In the bloodstream an unusually tight interaction between the bacteria and the brain microvasculature endothelial cells is established, leading to cortical plaque formation that results in opening of the blood brain barrier and bacterial invasion of the brain. This interaction is mediated by Type IV pili (T4P), long thin polymers of pilin proteins that interact with two endothelial cell receptors, CD147 and the β2 adrenergic receptor (β2AR). The interaction with CD147 is responsible for bacterial adhesion and the interaction with the β2AR induces signalling in endothelial cells. N. meningitidis PilE (Nm PilE) is 78% identical to Ng PilE and 100% identical in α1. Here we report the 1.44 Å X-ray crystal structure of Nm PilE and a cryoEM reconstruction of the Nm pilus at higher resolution, ∼6 Å, than any T4P structure reported previously.

The Iterative Helical Real Space Reconstruction (IHRSR)41 approach was used to obtain the reconstruction, which after sorting converged to a rise of 10.3 Å and a rotation of 100.8° for the subset of segments used. The cryoEM map, with an estimated resolution of ∼6 Å, shows well-defined density for the PilE globular domain, with a central depression and a protruding ridge on one side. Rod-like density is present in the core of the filament consistent with the protruding N-terminal α-helical segments of PilE, α1N. This density shows that the α1N segments are staggered in a helical array in the filament core and partially tilted relative to the filament axis, with their N termini close to the centre of the filament and their C termini lying at a larger radius. Thus, we built a model for the Nm T4P by separately fitting the Nm ΔN-PilE structure (residues 29–161) and α1N from the full-length Ng PilE structure, separated into two segments, α1:1–14 and α1:24–28, into the cryoEM map. These α-helical segments were then joined by an extended non-helical segment, α1:15–23. The ridge of density located on one side of the globular domain is occupied by the hypervariable segment of the D-region, the β-hairpin loop, β6 and the loop following β6, with Lys140 prominently displayed at its most protruding point. In our Nm T4P model the α1 segment 24–53 is curved but runs roughly parallel to the filament axis while α1:1-14 is tilted with its N terminus oriented toward the centre of the filament. This orientation places the side chain of Glu5 in close proximity (<5 Å) to the N-terminal amine of Phe1 (Phe1:N) on the neighbouring α1 in the 1-start helix, consistent with a salt bridge, which matches perfectly the well-defined channel connecting the rod-like densities at their termini. The cryoEM map shows that α1 is non-helical between the helix-breaking residues Gly14 and Pro22. The new Nm T4P model with its non-helical α1 segment provides a molecular basis with which to understand the reversible force-dependent polymorphism observed for both Nm and Ng T4P2932.

>[26x]FTLIELMIVIAIVGILAAVALPAYQDYTARAQVSEAILLAEGQKSAVTEYYLNHGEWPGDNSSAGVATSADIKGKYVQSVTVANGVITAQMASSNVNNEIKSKKLSLWAKRQNGSVKWFCGQPVTRTTATATDVAAANGKTDDKINTKHLPSTCRDDSSAS> MALNRI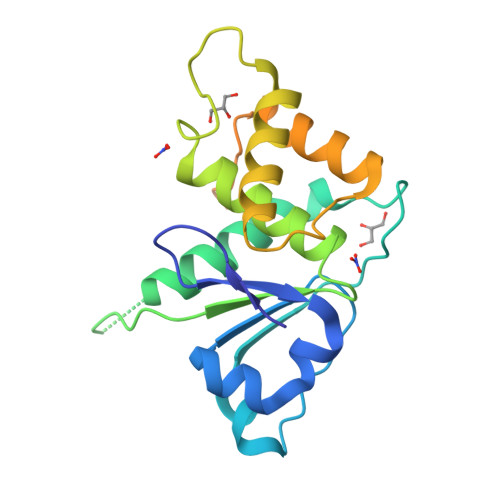KGDDELFVGGVFGANRARLIKEHRITHILSVIDHTVDRENEAFRHVKHLSIDIDDMEDQDILIHLPKIVRFIDSGLRGIDPSDSSAVASPGVVLVHCAMGKSRSVTAIIAYLLWKYPYRFGKSDPNISAKEAVSRALEWVRETRPIAGPNDGFMRQLEMWWDMGCPADSDDAVEREPAYQRWLYQREVEDAARIGRAPDRLRFEDEAATAEGSHHHHHH> FQRSTPAITLESPDIKYPLRLIDREIISHDTRRFRFALPSPQHILGLPVGQHIYLSARIDGNLVVRPYTPISSDDDKGFVDLVIKVYFKDTHPKFPAGGKMSQYLESMQIGDTIEFRGPSGLLVYQGKGKFAIRPDKKSNPIIRTVKSVGMIAGGTGITPMLQVIRAIMKDPDDHTVCHLLFANQTEKDILLRPELEELRNKHSARFKLWYTLDRAPE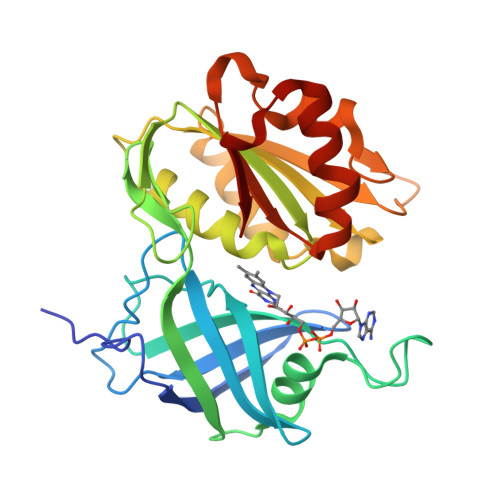AWDYGQGFVNEEMIRDHLPPPEEEPLVLMCGPPPMIQYACLPNLDHVGHPTERCFVF The atypical cadherins Fat and Dachsous are key regulators of cell growth and animal development. In contrast to classical cadherins, which form homophilic interactions to segregate cells, Fat and Dachsous cadherins form heterophilic interactions to induce cell polarity within tissues. Here, we determine the co-crystal structure of the human homologs Fat4 and Dachsous1 (Dchs1) to establish the molecular basis for Fat-Dachsous interactions. Fat4 and Dchs1 are two of the largest members of the cadherin superfamily and contain 34 and 27 extracellular cadherin (EC) domains, respectively.

The binding domains of Fat4 and Dchs1 form an extended interface along extracellular cadherin (EC) domains 1-4 of each protein. The Fat4 EC1–EC4 domains are positioned opposite the Dchs1 EC4, EC3, EC2, and EC1 domains, respectively. There were direct contacts between Fat4(EC1):Dchs1(EC4), Fat4(EC2):Dchs1(EC3), and Fat4(EC4):Dchs1(EC1), but no substantial contacts were observed between Fat4(EC3) and Dchs1(EC2). The Fat4(EC1):Dchs1(EC4) interface was oriented similarly to the Fat4(EC4):Dchs1(EC1) interface with one notable difference. The equivalent position of Leu379 for Fat4(EC4) is Arg387 in Dchs1(EC4), and this arginine forms a salt bridge with Glu120. The presence of an arginine at this position makes the Fat4(EC1):Dchs1(EC4) interface less hydrophobic than the Fat4(EC4):Dchs1(EC1) interface, and we speculate that this difference may be linked to the reduced contribution of Fat4(EC1):Dchs1(EC4) to the binding affinity. Within Dchs1(EC4), the Arg387 residue central to the Fat4-binding interface is highly conserved across all species sampled. Thus, the EC4 domain of Fat4 is indispensable for binding to Dchs1 while the EC4 of Dchs1 makes a minor contribution to the interaction. The alignment of EC2–EC3 of each protein revealed that the EC1 of Dchs1 is tilted by ~35° towards Fat4, making it the only protomer that adopts such a pronounced curvature in a protocadherin-like binding interface. This distinctive conformation was observed in both the high- and low-resolution structures.

> PQAGSLDLQIDEEQPAGTLIGDISAGLPAGTAAPLMYFISAQEGSGVGTDLAIDEHSGVVRTARVLDREQRDRYRFTAVTPDGATVEVTVRVADINDHAPAFPQARAALQVPEHTAFGTRYPLEPARDADAGRLGTQGYALSGDGAGETFRLETRPGPDGTPVPELVVTGELDRENRSHYMLQLEAYDGGSPPRRAQALLDVTLLDINDHAPAFNQSRYHAVVSESLAPGSPVLQVFASDADAGVNGAVTYEINRRQSEGDGPFSIDAHTGLLQLERPLDFEQRRVHELVVQARDGGAHPELGSAFVTVHVRDANDNQPSMTVIFLSADGSPQVSEAAPPGQLVARISVSDPDDGDFAHVNVSLEGGEGHFALSTQDSVIYLVCVARRLDREERDAYNLRVTATDSGSPPLRAEAAFVLHV;> MDLAPDRATGRPWLPLHTLSVSQLLRVFWLLSLLPGQAWVHGAEPRQVFQVLEEQPPGTLVGTIQTRPGFTYRLSESHALFAINSSTGALYTTSTIDRESLPSDVINLVVLSSAPTYPTEVRVLVRDLNDNAPVFPDPSIVVTFKEDSSSGRQVILDTATDSDIGSNGVDHRSYRIIRGNEAGRFRLDITLNPSGEGAFLHLVSKGGLDREVTPQYQLLVEVEDKGEPKRRGYLQVNVTVQDINDNPPVFGSSHYQAGVPEDAVVGSSVLQVAAADADEGTNADIRYRLQDEGTPFQMDPETGLITVREPLDFEARRQYSLTVQAMDRGVPSLTGRAEALIQLLDVNDNDPVVKFRYFPATSRYASVDENAQVGTVVALLTVTDADSPAANGNISVQILGGNEQRHFEVQSSKVPNLSLIKVASALDRERIPSYNLTVSVSDNYGAPPGAAVQARSSVASLVIFVND1,2,3,4,5,6-HEXAHYDROXY-CYCLOHEXANE | C6 H12 O6 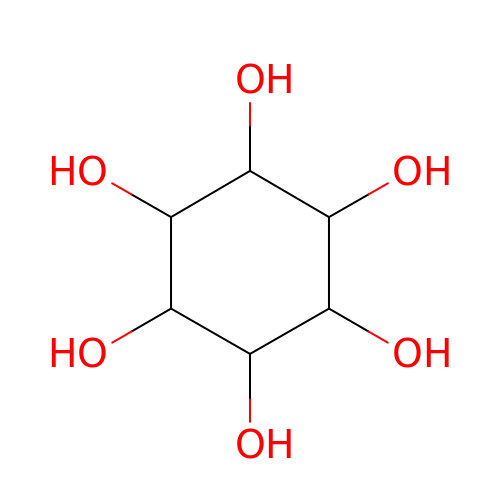| CDAISMWEOUEBRE-GPIVLXJGSA-N> MATLFIADLHLQTEEPEITAGFLRFLQGEARQADALYILGDLFEAWIGDDDPNPLHQQIASAIKAVVDAGVPCYFIHGNRDFLVGQRFARQSGMILLAEEERLDLYGREVLIMHGDTLCTDDQGYLAFRAKVHTPWIQRLFLALPLFIRHRIAARMRADSKAANSSKSMEIMDVNPQAVVDAMERHHVQWLIHGHTHRPAVHELQANGQPAWRVVLGAWHSEGSMVKVTPDDVELIHFPFHHHHHH

The LpxH enzyme cleaves the pyrophosphate bond of UDP-2, 3-bis(3-hydroxytetradecanoyl)-glucosamine (UDP-DAGn) to yield lipid X (PubChem CID 123907) and UMP in the fourth step of lipid A biosynthesis. Roughly 70% of Gram-negative bacteria, including the WHO critical priority Gram-negative pathogens for R&D of new antibiotics, utilize this enzyme. The importance of LPS, and lipid A in particular, for the viability and virulence of Gram-negative bacteria makes the inhibition of lipid A biosynthesis a promising target for the development of antibiotics. To enable a structure-based drug design approach for the optimization of JEDI-1444, we produced LpxH proteins from E. coli (EcLpxH) and K. pneumoniae (KpLpxH) and solved the X-ray crystal structures of various enzyme-product and inhibitor complexes during the optimization of the chemical series.

Since the pocket accommodating ring 1 is very lipophilic, the introduction of polarity here while retaining good target affinity was a challenging task. Optimization of the π–π stacking interactions between ring 1 and Phe141 led to a library of substituted heteroaromatic compounds. As expected, the introduction of polarity here was a trade-off between lipophilicity and target binding. Nevertheless, to our satisfaction, many analogs showed significant improvements in serum MIC. The best compound in this group, EBL-3339, showed only minor reduction in MIC activity upon the addition of serum while retaining good target affinity. The X-ray structure of the complex of EBL-3647 with KpLpxH shows that it retains the binding mode of the original hit compound JEDI-1444 (as well as EBL-3339), with both protein and ligand closely superimposable.5,5-dimethyl-7-[(1~{S})-4-oxidanyl-1~{H}-inden-1-yl]-2-phenylazanyl-pyrrolo[2,3-d]pyrimidin-6-one | C23 H20 N4 O2 | 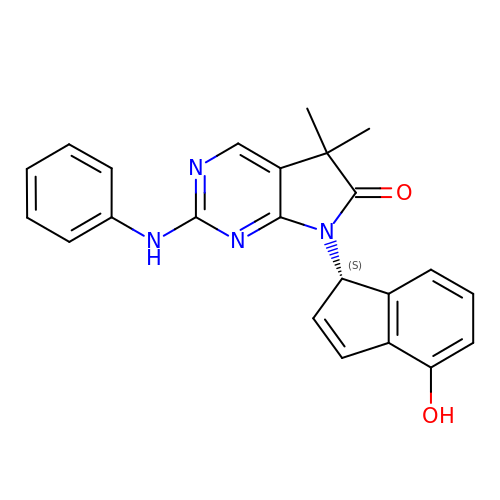XYYZSCWSVMFLOM-SFHVURJKSA-N>[2x]MRMDEF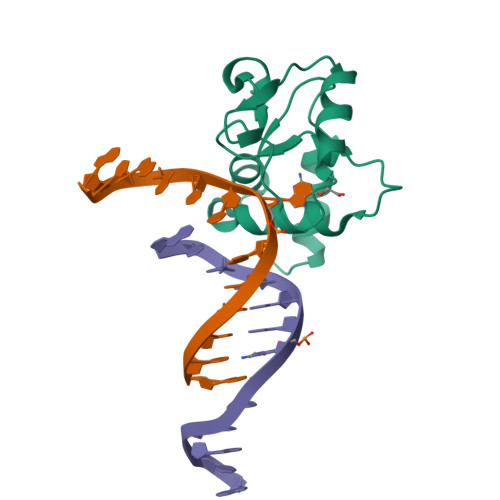YTKVYDAVCEIPYGKVSTYGEIARYVGMPSYARQVGQAMKHLHPETHVPWHRVINSRGTISKRDISAGEQRQKDRLEEEGVEIYQTSLGEYKLNLPEYMWKPGSHHHHHH>MAHHHHHHVGTGSNDDDDKSPDPNWELVYTARLQMVKVLAVLYDGGEHAKQVPGLLGTTENELGLRKWLEDQGHTLVTTSDKDREGSTFDRELEDAEIIITTPFHPGYLTAERLARAKKLKLAVTAGIGSDHVDLDAANKTNGGITVAEV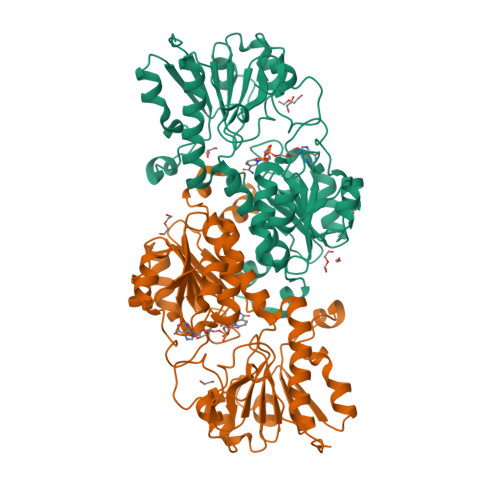TGSNVVSVAEHVVMTILVLVRNFVPAHEQIEAGRWDVAEVAKDEYDLEGKVVGTVGVGRIGERVLRRLKGFDCKELLYYDYQPLSPEKEKEIGCRRVENLEEMLAQCDVVTINCPLHESTRGLFNKDLISKMKRGSWLVNTARGAIVVKEDVAEALRTGHLRGYGGDVWFPQPAPADHVLRTAKNPFGGGNAMVPHMSGTSLDAQKRYAEGVKRILDSYLSGRFDYRPEDLIVHQGKYATRAYGQREDVKIPGQHHHHHH[4x]>AGGHGDVGMHVKEKEKNKDENKRKDEERNKTQEEHLKEIMKHIVKIEVKGEEAVKKEAAEKLLEKVPSDVLEMYKAIGGKIYIVDGDITKHISLEALSEDKKKIKDIYGKDALLHEHYVYAKEGYEPVLVIQSSEDYVENTEKALNVYYEIGKILSRDILSKINQPYQKFLDVLNTIKNASDSDGQDLLFTNQLKEHPTDFSVEFLEQNSNEVQEVFAKAFAYYIEPQHRDVLQLYAPEAFNYMDKFNEQEINLSLEELKDQRMLSRYEKWEKIKQHYQHWSDSLSEEGRGLLKKLQIPIEPKKDDIIHSLSQEEKELLKRIQIDSSDFLSTEEKEFLKKLQIDIRDSLSEEEKELLNRIQVDSSNPLSEKEKEFLKKLKLDIQPYDINQRLQDTGGLIDSPSINLDVRKQYKRDIQNIDALLHQSIGSTLYNKIYLYENMNINNLTATLGADLVDSTDNTKINRGIFNEFKKNFKYSISSNYMIVDINERPALDNERLKWRIQLSPDTRAGYLENGKLILQRNIGLEIKDVQIIKQSEKEYIRIDAKVVPKSKIDTKIQEAQLNINQEWNKALGLPKYTKLITFNVHNRYASNIVESAYLILNEWKNNIQSDLIKKVTNYLVDGNGRFVFTDITLPNIAE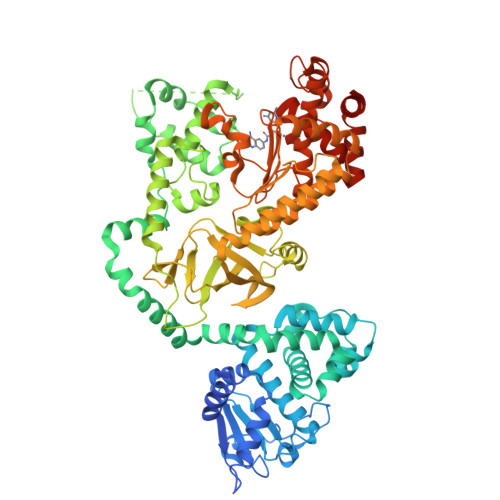QYTHQDEIYEQVHSKGLYVPESRSILLHGPSKGVELRNDSEGFIHEFGHAVDDYAGYLLDKNQSDLVTNSKKFIDIFKEEGSNLTSYGRTNEAEFFAEAFRLMHSTDHAERLKVQKNAPKTFQFINDQIKFIINS[2x]> PLFN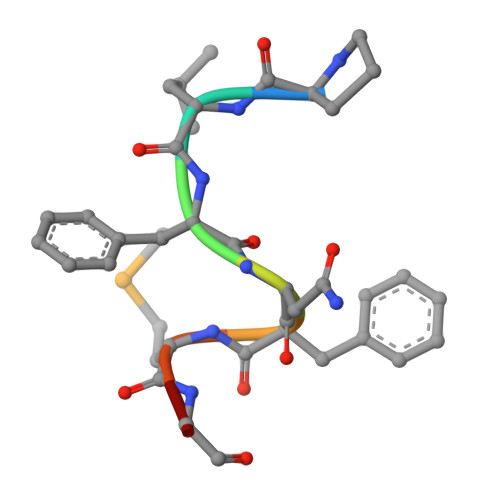FMGC>MGSDKIHHHHHHMMGLKAHAMVLEKFNQPLVYKEFEISDIPRGSILVEILSAGVCGSDVHMFRGEDPRVPLPIILGHEGAGRVVEVNGEKRDLNGELL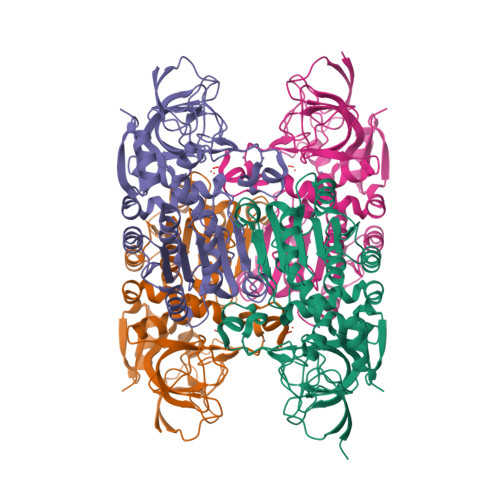KPGDLIVWNRGITCGECYWCKVSKEPYLCPNRKVYGINRGCSEYPHLRGCYSSHIVLDPETDVLKVSEKDDLDVLAMAMCSGATAYHAFDEYPESFAGKTVVIQGAGPLGLFGVVIARSLGAENVIVIAGSPNRLKLAEEIGADLTLNRRETSVEERRKAIMDITHGRGADFILEATGDSRALLEGSELLRRGGFYSVAGVAVPQDPVPFKVYEWLVLKNATFKGIWVSDTSHFVKTVSITSRNYQLLSKLITHRLPLKEANKALELMESREALKVILYPEG[4x]>[6x]HPETLVKVKDAEDQLGARVGYIELDLNSGKILESFRPEERFPMMSTFKVLLCGAVLSRIDAGQEQLGRRIHYSQND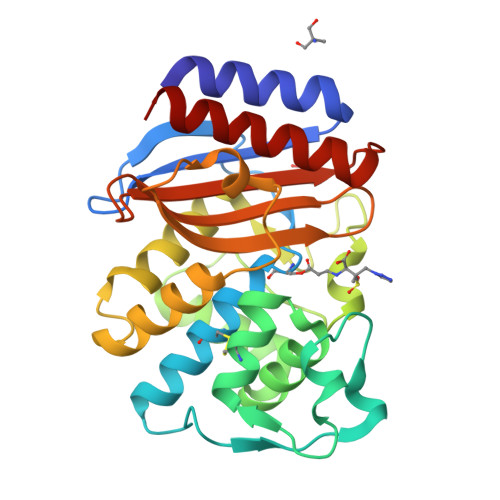LVEYSPVTEKHLTDGMTVRELCSAAITMSDNTAANLLLTTIGGPKELTAFLHNMGDHVTRLDRWEPELNEAIPNDERDTTMPAAMATTLRKLLTGELLTLASRQQLIDWMEADKVAGPLLRSALPAGWFIADKSGAGERGSRGIIAALGPDGKPSRIVVIYTTGSQATMDERNRQIAEIGASLIKHW> GIDELYKKEFGIVAGVDEAGRGCLAGPVVAAAVVLEKEIEGINDSKQLSPAKRERLLDEIMEKAAVGIGIASPEEIDLYNIFNATKLAMNRALENLSVKPSFVLVNGKGIELSVPGTCLVKGDQKSKLIGAASIVAKVFRDRLMSEFHRMYPQFSFHKHKGYATKEHLNEIRKNGVLPIHRLSFEPVLELLTDDLLREFFEKGLISENRFERILNLLGARKS

Ribonucleases H are the only known enzymes that degrade the RNA strand of RNA/DNA hybrids in a sequence-nonspecific manner, and therefore are essential for DNA integrity. Type 1 enzymes hydrolyze all types of RNA/DNA hybrids but require at least four ribonucleotides embedded in a dsDNA sequence to cleave (Ohtani et al., 1999), while most type 2 enzymes can hydrolyze all types of hybrids including DNA-RNA1-DNA/DNA (Eder and Walder, 1991; Eder et al., 1993; Jeong et al., 2004; Ohtani et al., 1999, 2008). Tm-RNase H2 contains two domains—the N-terminal catalytic core adopts the RNase H fold. The nucleic acid substrate is bound in a groove on the surface of the protein which is formed between the catalytic and the C-terminal domains.

For the initial crystallization trials, we employed an inactive Tm-RNase H2 D107N protein. Tm-RNase H2 ΔC D107N underwent extensive crystallization experiments in the presence of RNA/DNA hybrids of various lengths and 12 bp dsDNA harboring a single ribonucleotide in one of the strands (DNA5-RNA1-DNA6/DNA12). Protein-nucleic acid complex crystals were obtained only for the latter substrate, and they grew in the presence of 0.3 M MgCl2. The complex structure was solved by molecular replacement method with the apo structure solved at JCSG as a search model and subsequent manual modeling of the nucleic acid. We call this structure 1R-Mg, and it was refined to 2.0 Å resolution. Ions A and C were also observed in structures of mutant Tm-RNase H2 D107N solved with Mg2+ (structure 1R-Mg), Mn2+ (structure 1R-Mn), and Ca2+ (data not shown), but metal ion B was missing in all these structures. Therefore, the lack of binding of ion B does not depend on its identity and is likely caused by D107N mutation. The 5′-phosphate of the ribonucleotide of the (5′)RNA-DNA(3′) junction is located at the active site of the enzyme in agreement with the cleavage preference. The aromatic ring of the tyrosine stacks with the deoxyribose ring of the deoxyribonucleotide at the +2 position (numbering relative to the scissile phosphate) and seems to push it up, leading to deformation of the nucleic acid backbone at the (5′)RNA-DNA(3′) junction located between positions +1 and +2. The nonbridging oxygen-metal ion distance is 3.3 Å for Mn2+ ion versus 2.4 Å for Mg2+.> DEFQWKGLPVVKSGLDVGGMPTGTRYHRSPAWPEEQPGETHAPAPFGSGDKRYTFSQTEMLVNGLKPYTEPTAGVPPQLLSRAVTHVRSYIETIIGTHRSPVLTYHQACELLERTTSCGPFVQGLKGDYWDEEQQQYTGVLANHLEQAWDKANKGI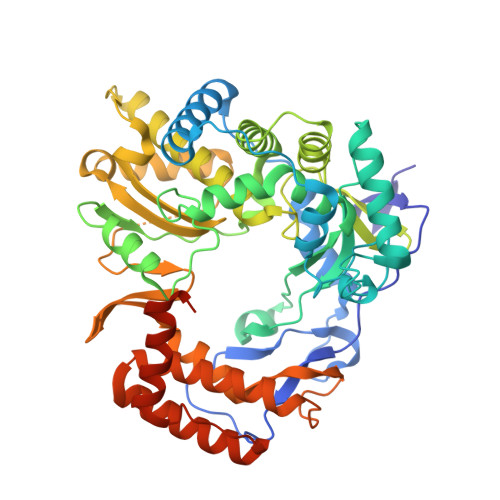APRNAYKLALKDELRPIEKNKAGKRRLLWGCDAATTLIATAAFKAVATRLQVVTPMTPVAVGINMDSVQMQVMNDSLKGGVLYCLDYSKWDSTQNPAVTAASLAILERFAEPHPIVSCAIEALSSPAEGYVNDIKFVTRGGLPSGMPFTSVVNSINHMIYVAAAILQAYESHNVPYTGNVFQVETIHTYGDDCMYSVCPATASIFHTVLANLTSYGLKPTAADKSDAIKPTNTPVFLKRTFTQTPHGIRALLDITSITRQFYWLKANRTSDPSSPPAFDRQARSAQLENALAYASQHGPVMFDTVRQIAIKTAQGEGLVLVNTNYDQALATYNAWFIGGTVPDPVGHTEGTHKIVFEME>[2x]SMARAPPYQEPPWGGPAT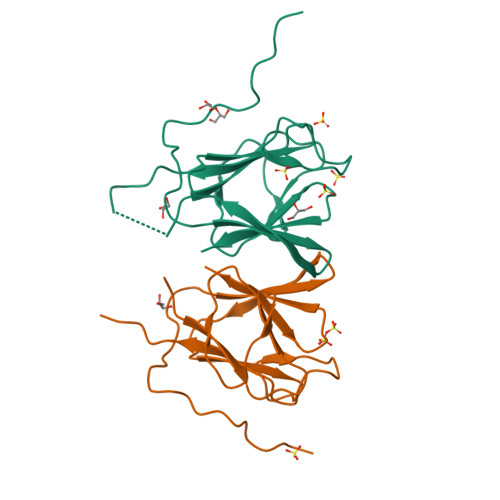APYSLETLKGGTILGTRSLKGTSYCLFGRLSGCDVCLEHPSVSRYHAVLQHRASGPDGECDSNGPGFYLYDLGSTHGTFLNKTRIPPRTYCRVHVGHVVRFGGSTRLFILQG> GGGTTAGG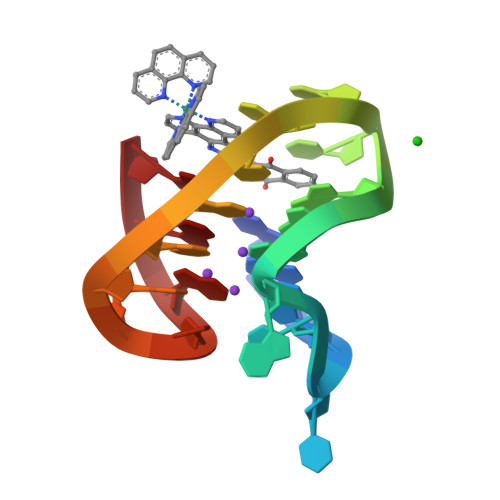GTTAGGGTTTGGG5-(1-methylindol-3-yl)pyrimidin-4-amine | C13 H12 N4 | 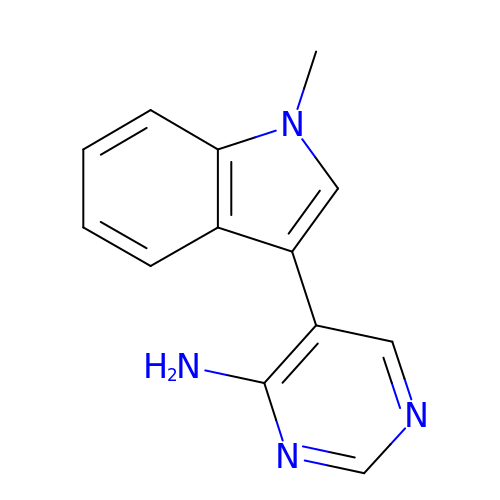IQUSYKXSEAUSFE-UHFFFAOYSA-N>ERVSFQPFYPKTEKPNRPQRF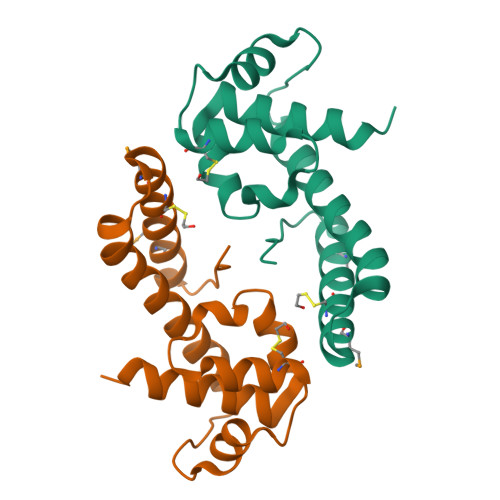AHVSSAPSLEFLEKLVIRYLLEDRSLLDLAVGYIHSGVFLHKKQEFDALCQEKLDDPKLVALLLDANLPLKKGGFEKELRLLILRYFERQLKEIPKSSLPFSEKMICLKKARQAIMKLKQGELVAILEHHHHHH[2x]> MGFETVVPAPPTRDDELRMIKATEEQFLQQPRYKLYMNEAHRIAKMNHGDRHNNIRAHFWSNFALGLLITGPIFIIP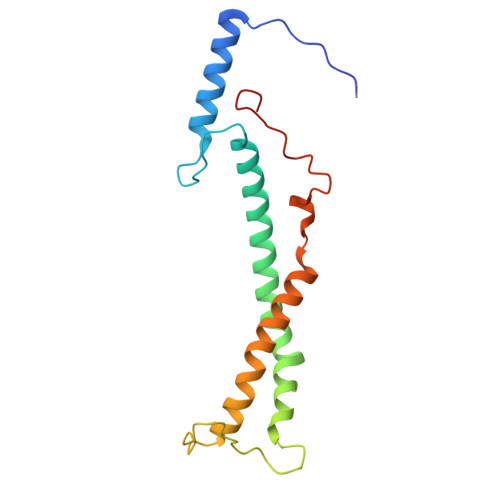FGKAFRNLRSGVPYYFRPKYVFTQKNQYNQDRNWGAMKKQIPLWLGLSTAYAYWFTDFSINDDEWLEKGKVIYPHQTIKVL> MNDCDEKN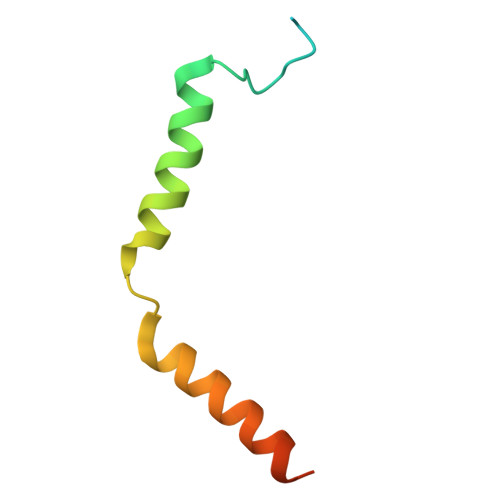LTNHFTFGDDLLGVNSEIARKLRQFYLEIQEEALPARLLELLERLEQAERFGLNNAEKV> MSHYALSPEHKQMVEGHLAETDPEVNQIIKDEVDRQKHSIVLIASENFTSTSVFDALGTPMCNKYSEGYPGARYYGGNEHIDRMEILCQQRALKAFHLDGSRWGVNVQTLSGSPANLQVYQAIMKPHDRLMGLDLPHGGHLSHGYQTDTRKISAVSTYFETMPYRVDLETGIIDYDMLEKTAVLYRPKVLVAGTSAYCRLIDYKRMREIADKVGAYLVVDMAHISGLIAAGVIPSPFEYADIVTTTTHKSLRGPRGAMIFFRKGVRSVNPKTGKEIYYDLENPINFSVFPGHQGGPHNHTIAALATALKQAATPEFKQYQEQVLK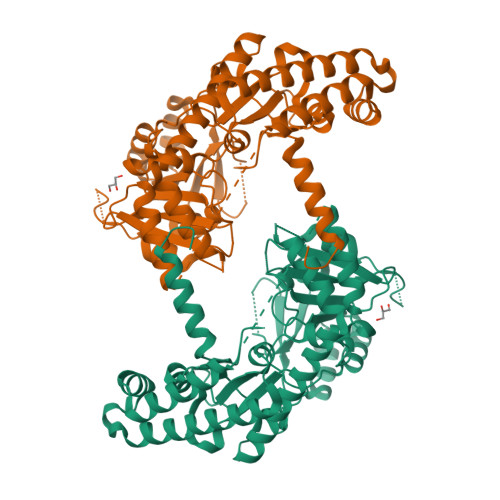NAKALENEFKRLGYKLVSDGTDSHMVLVSLKDKDIDGARIETVCENINIALNKNSIPGDRSALVPGGVRIGAPAMTTRGASEEDFVKIANYIDKSVQYAKKVQSELPIEANKLKDFKAKIAEGSDEITQLKNEISAWAGEFPLSV~{N}-[[2-methyl-4-[2-[(1-methylpyrazol-4-yl)amino]pyrimidin-4-yl]phenyl]methyl]-3-propan-2-yloxy-azetidine-1-carboxamide 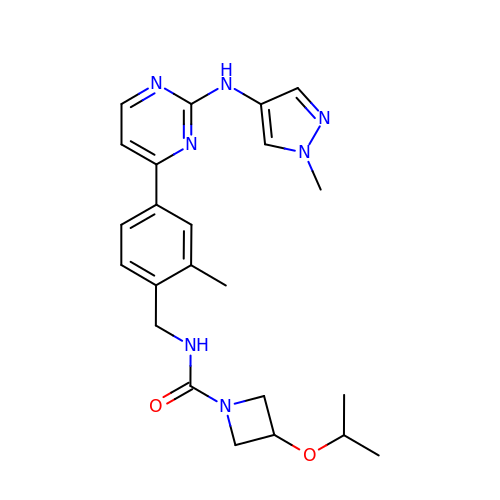| C23 H29 N7 O2 | BMWMKGNVAMXXCH-UHFFFAOYSA-N> AGRPAVSASSRWLEGIRKWYYNAAGFNKYGLMRDDTIYENDDVKEA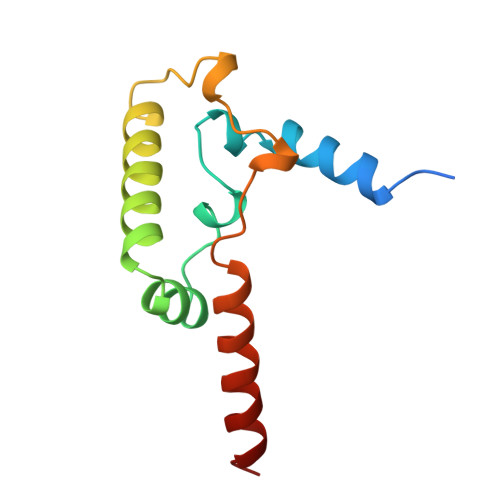IRRLPENLYDDRMFRIKRALDLNMRQQILPKEQWTKYEEDVPYLEPYLKEVIRERKEREEWDK>[3x]GSAMGSDTVIDEKINIPVPLGTVFSLLYGDDTSYIKKIIENQNNFNVCDIPKFVNNAREITYTKKLNNSFGPKQTKCIVTETIEHMDLNSFFMVKQIVRSPDVPYGSSFSVHTRFFYSW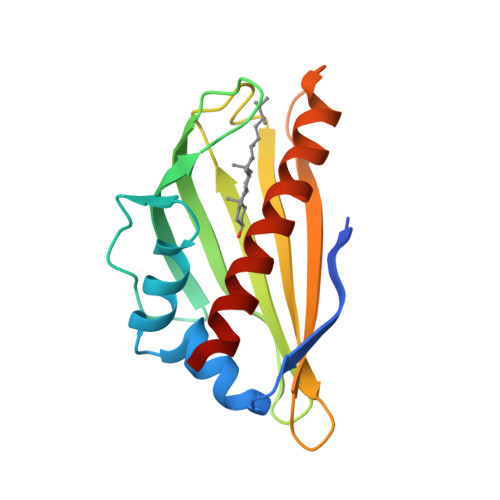GDHNTTNMKVVTNVVWTGKSMLKGTIEKGSIDGQRSSTKQLVDDLKKIISN>[2x]SNAMAGGDRGSGGTGNVRRLVIVESPTKARKIAGYLGSNYVVESSRGHIRDLPRNAADVPAKFKSEPWARLGVNVDQNFEPLYIVSPEKKSTVTELKGLLKDVDELYLATDGDREGEAIAWHLLETLKPRVPVKRMVFHEITEPAIRNAAENPRDLDIALVDAQETRRILDRLYG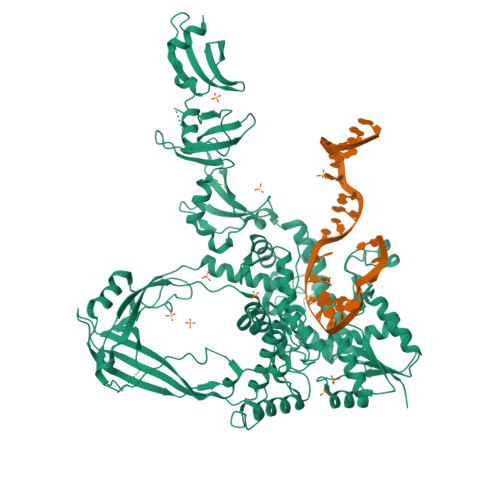YEVSPVLWKKVAPKLSAGRVQSVATRIIVQRERERMAFHSASYWDVTAELDASVSDPSASPPKFTAKLNTVDGRRVATGRDFDSLGQLKRPDEVLVLDEASAGALASGLRGAQLAVTSVEQKPYTRRPYAPFMTSTLQQEAARKLRFSSERTMSIAQRLYENGYITYMRTDSTTLSESAINAARTQARQLYGEEYVHPSPRQYTRKVKNAQEAHEAIRPAGDVFQTPGQLHSALDTDEFRLYELIWQRTVASQMADARGTTLSLRIGGSASSGEQVVFNASGRTITFPGFLKAYVESIDELAGGESDDAESRLPNLTQGQRVDAADLSADGHQTSPPARYTEASLIKALEELGIGRPSTYSSIIKTIQDRGYVQKKGSALVPSWVAFAVVGLLEQHFGRLVDYDFTAAMEDELDEIANGQEQRTNWLNNFYFGGEHGVEGSIARAGGLKQLVGGNLEGIDAREVNSIKVFDDSEGRPVYVRVGRNGPYLERMVDDPDNPGEQKPQRANLKEDLTPDELTPELAEKLFATPQEGRSLGIDPETGHEIVAKDGRFGPYVTEVLPEPEDGGDDGTAGTPAKKGKKPTGPKPRTGSLFRSMDLETVTLEDALKLLSLPRVVGVDPTTNEEITAQNGRYGPYLKRGTDSRSLATEDQIFTITLDEALKIYAE> MIPQTLTNTNLFIDGVSFAGDVPSLTLPKLAVKTEQYRAGGMDAPVSIDMGLEAMEAKFSTNGARREALNFFGLADQSAFNGVFRGS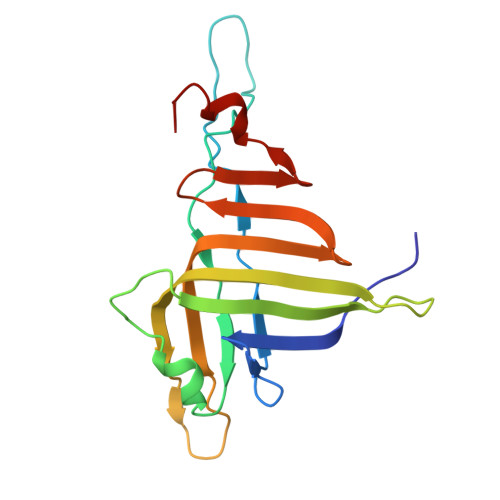FKGQKGASVPVVATLRGLLKEVDPGDWKAGEKAEFKYAVAVSYYKLEVDGREVYEIDPVNGVRAINGVDQLAGMRNDLGL[(3S,4R)-4-(thiophen-3-yl)pyrrolidin-3-yl]methanol 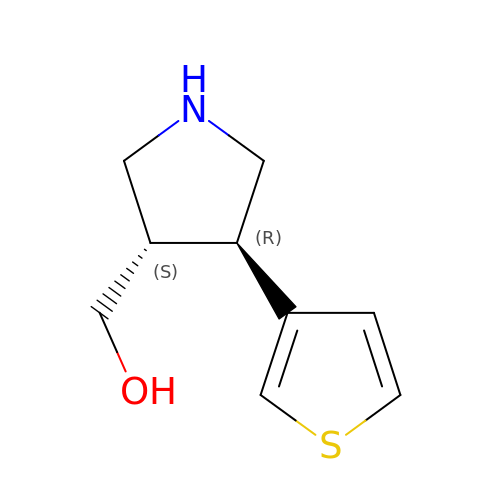| C9 H13 N O S | SWXORFHOLPJLTG-IUCAKERBSA-N6-(2,6-DICHLORO-PHENYL)-8-METHYL-2-(3-METHYLSULFANYL-PHENYLAMINO)-8H-PYRIDO[2,3-D]PYRIMIDIN-7-ONE 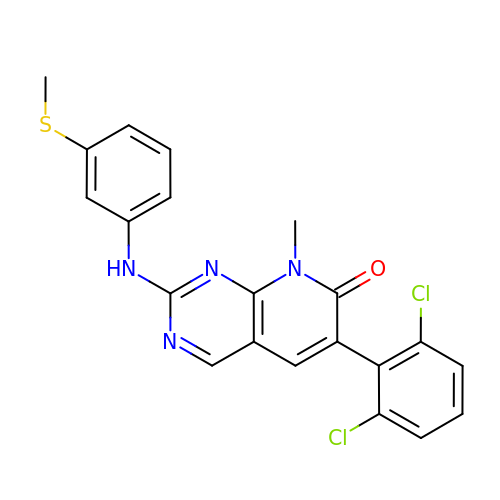| C21 H16 Cl2 N4 O S | VAARYSWULJUGST-UHFFFAOYSA-N2-acetamido-6-fluorobenzoic acid | C9 H8 F N O3 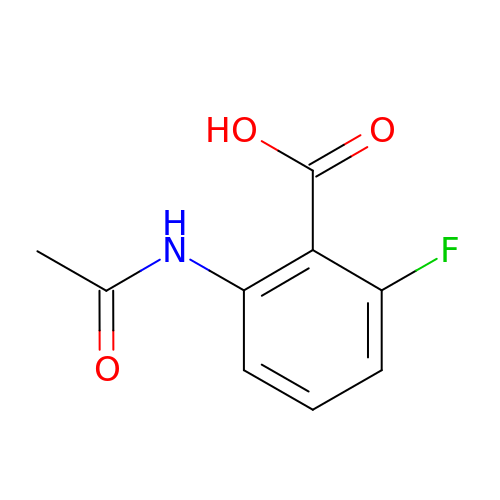| IWTHKNXLQDASPO-UHFFFAOYSA-N>MRGSHHHHHHSNFAIILAAGKGTRMKSDLPKVLHKVAGISMLEHVFRSVGAIQPEKTVTVVGHKAELVEEVLAGQTEFVTQSEQLGTGHAVMMTEPILEGLSGHTLVIAGDTPLITGESLKNLIDFHINHKNVATILTAETDNPFGYGRIVRNDNAEVLRIVEQKDATDFEKQIKEINTGTYVFDNERLFEALKNINTNNAQGEYYITDVIGIFRETGEKVGAYTLKDFDESLGVNDRVALATAESVMRRRINHKHMVNGVSFVNPEATYIDIDVEIAPEVQIEANVILKGQTKIGAETVLTNGTYVVDSTIGAGAVITNSMIEESSVADGVTVGPYAHIRPNSSLGAQVHIGNFVEVKGSSIGENTKAGHLTYIGNCEVGSNVNFGAGTITVNYDGKNKYKTVIGDNVFVGSNSTIIAPVE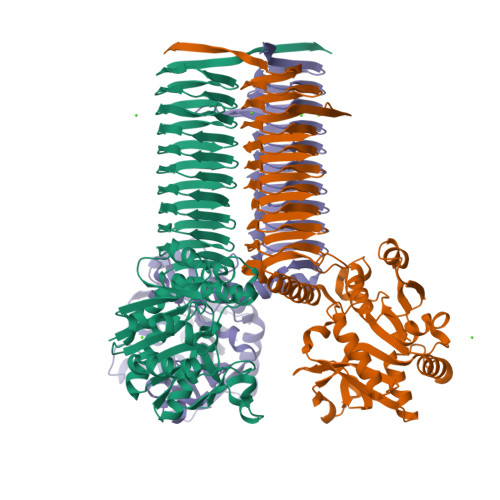LGDNSLVGAGSTITKDVPADAIAIGRGRQINKDEYATRLPHHPKNQ[2x]> GPLGSLCGRVFKVGEPTYSCRDCAVDPTCLLCMECFLGSIHRDHRYRMTTSGGGGFCDCGDTEAWKEGP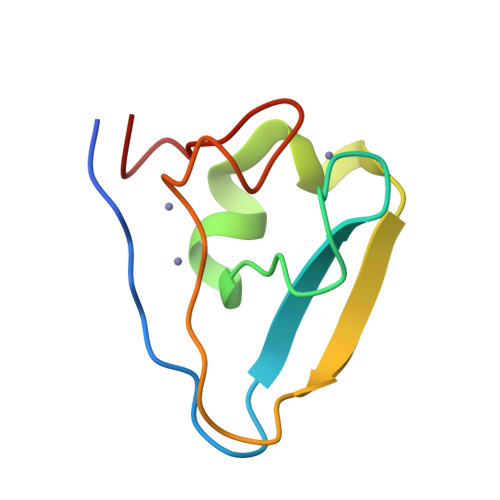YCQKHE PCNA is a ring-shaped homotrimeric protein, with each subunit consisting of two domains connected by a flexible linker called the inter-domain connecting loop (IDCL). CAF-1 association with replicating DNA, and the targeting of newly synthesized histones to sites of DNA replication and repair requires its interaction with proliferating cell nuclear antigen (PCNA), the eukaryotic sliding clamp that acts as a processivity factor for polymerases during DNA synthesis. Recruitment of PCNA-interacting proteins to replication forks is generally mediated by a conserved sequence in these proteins called a PCNA-interacting protein (PIP) motif that interacts with PCNA in a region between the two domains on a single subunit near the IDCL. In this study, we focused on three separation-of-function amino acid substitutions in PCNA that cause defective gene silencing and exhibit reduced CAF-1 association with chromatin in vivo, as well as inhibit binding to CAF-1 in vitro partially or completely (D41A/D42A, R61A/D63A, and L126A/I128A).

The X-ray crystal structure of the L126A/I128A mutant PCNA protein was determined to a resolution of 1.93 Å. The L126A/I128A residues are located within the IDCL of PCNA, which is directly above the canonical PIP-interacting region. Compared to the wild-type structure, there are significant backbone changes in the structure of the L126A/I128A mutant PCNA in the IDCL. The α carbons of residues 123 to 129 have moved from 1.8 to 2.9 Å relative to their positions in the wild-type PCNA structure. Similarly, there are significant backbone changes in the structure of the mutant PCNA protein in loop B, which is more than 15 Å from the substitutions. Finally, there are significant backbone changes in the structure of the mutant PCNA protein in loop D, which is approximately 15 Å from the substitutions. The α carbons of residues 41 to 44 have moved from 1.5 to 2.7 Å relative to their positions in the wild-type PCNA structure. In the structure of the L126A/I128A mutant protein, we observe clear electron density in the vicinity of the IDCL, loop B, and loop D into which we modeled a portion of a PEG molecule and a chloride ion from the crystallization conditions. To our knowledge, binding of small molecule ligands at this site has not previously been observed with PCNA. Of the three mutant proteins crystallized, the L126A/I128A substitutions cause the most dramatic changes to this surface cavity compared to the wild-type protein.

> MHHHHHHMLEAKFEEASLFKRIIDGFKDCVQLVNFQCKEDGIIAQAVDDSRVLLVSLEIGVEAFQEYRCDHPVTLGMDLTSLSKILRCGNNTDTLTLIADNTPDSIILLFEDTKKDRIAEYSLKLMDIDADFAKAEELQYDSTLSLPSSEFSKIVRDLSQLSDSINIMITKETIKFVADGDIGSGSVIIKPFVDMEHPETSIKLEMDQPVDLTFGAKYLLDIIKGSSLSDRVGIRLSSEAPALFQFDLKSGFLQFFLAPKFNDEE>[12x]MTSFTIPGLSDKKASDVADLLQKQLSTYNDLHLTLKHVHWNVVGPNFIGVHEMIDPQVELVRGYADEVAERIATLGKSPKGTPGAIIKDRTWD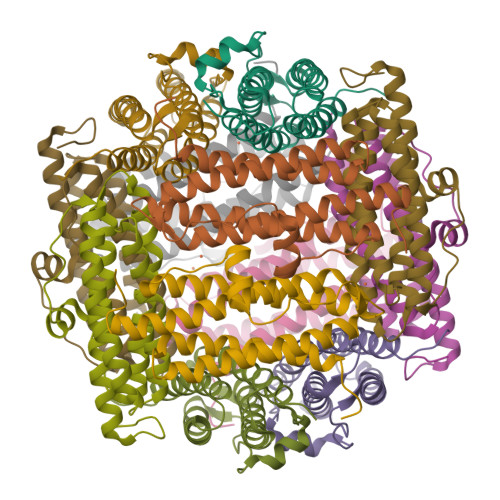DYSVERDTVQAHLAALDLVYNGVIEDTRKSIEKLEDLDLVSQDLLIAHAGELEKFQWFVRAHLESAGGQLTHEGQSTEKGAADKARRKSA>MLQPECSRSEEDLSDEKERKWEQLSRHWHTVVLASSDRSLIEEEGPFRNFIQNITVESGNLNGFFLTRKNGQCIPLYLTAFKTEEARQFKLNYYGTNDVYYESSKPNEYAKFIFYNYHDGKVNVVANLFGRTPNLSNEIKKRFEEDFM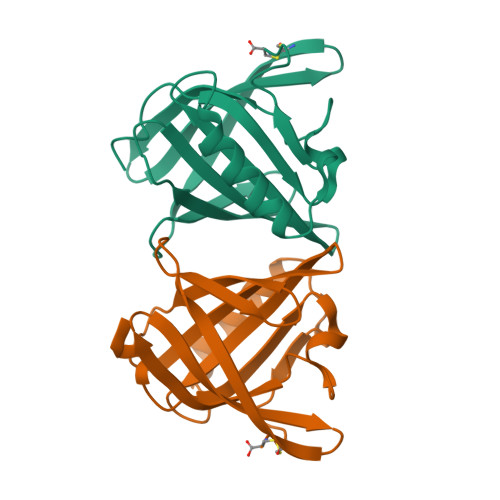NRGFRRENILDISEVDHC[4x]>AALEPTDSGAPSAIVMFPVGEKPNPKGAAMKPVVFNHLIHEKKIADCETCHHTGDPVSCSTCHTVEGKAEGDYITLDRAMHATDIAARAKGNTPTSCVSCHQSETKERRECAGCHAITTPKDDEAWCATCHDITPSMTPSEM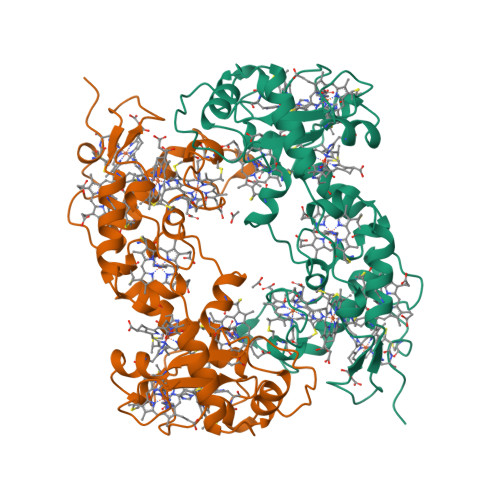QKGIAGTLLPGDNEALAAETVLAEATVAPVSPMLAPYKVVIDALADKYEPSDFTHRRHLTSLMESIKDDKLAQAFHDKPEILCATCHHRSPLSLTPPKCGSCHTKEIDAADPGRPNLMAAYHLECMGCHKGMAVARPRDTDCTTCHKAAA[2x]> MGKTNDWLDFDQLAEEKVRDALKPPSMYKVILVNDDYTPMEFVIDVLQKFFSYDVERATQLMLAVAYQGKAICGVFTAEVAETKVAMVNKYARENEHPLLCTLEKA;> MLNQE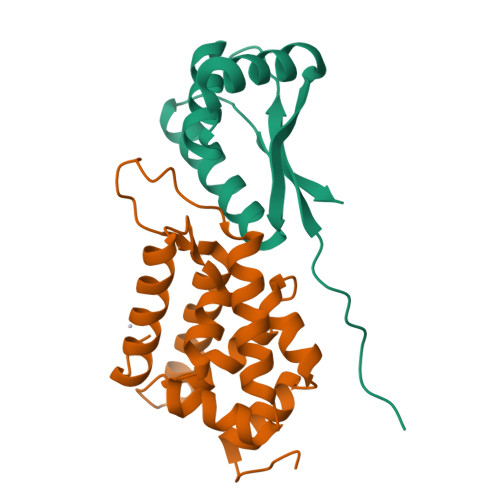LELSLNMAFARAREHRHEFMTVEHLLLALLSNPSAREALEACSVDLVALRQELEAFIEQTTPVLPASEEERDTQPTLSFQRVLQRAVFHVQSSGRNEVTGANVLVAIFSEQESQAAYLLRKHEVSRLDVVNFISHGTRKDE(2S)-2-[4-(cyclopropylsulfonyl)-1H-indazol-1-yl]-N-(5-fluoro-1,3-thiazol-2-yl)-3-(oxan-4-yl)propanamide | C21 H23 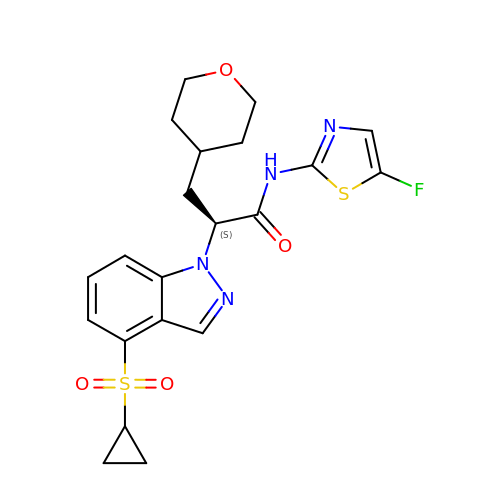F N4 O4 S2 | VFUKAAVEACENGY-KRWDZBQOSA-N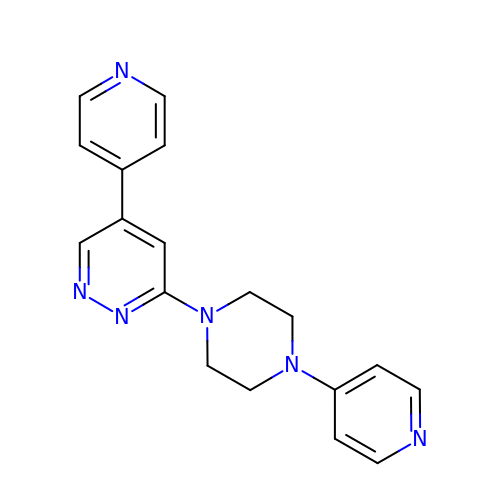5-(pyridin-4-yl)-3-[4-(pyridin-4-yl)piperazin-1-yl]pyridazine | C18 H18 N6 | PMYQZDHMSFEWMS-UHFFFAOYSA-N>[2x]MPFTYSIEATRNLATTERCIQDIRNAPVRNRSTQFQLAQQNMLAYTFGEVIPGFASAGINGMDYRDVIGRPVENAVTEGTHFFRDDFRVDSNAKAKVAGDIFEIVSSAVMWNCAARWNSLMVGEGWRSQPRYSRPTLSPSPRRQVAVLNLPRSFDWVSLLVPESQEVIEEFRAGLRKDGLGLPTSTPDLAVVVLPEEFQNDEMWREEIAGLTRPNQILLSGAYQRLQGRVQPGEISLAVAFKRSLRSDRLYQPLYEANVMQLLLEGKLGAPKVEFEVHTLAPEGTNAFVTYEAASLYGLAEGRSAVHRAIRELYVPPTAADLARRFFAFLNERMELVNGENLYFQSHHHHHH

For the filament-forming sequence-specific DNA endonuclease SgrAI, the process of filamentation both accelerates its DNA cleavage activity and expands its DNA sequence specificity, thus allowing for many additional DNA sequences to be rapidly cleaved. Under basal conditions, SgrAI is a homodimeric and sequence-specific restriction endonuclease of 74 kDa with two active sites, one in each subunit. Each active site cleaves bound duplex DNA containing any one of 17 different 8 bp recognition sites. Three of these sites, known as primary sequences or primary sites, have the pattern CRCCGGYG (where R = A or G and Y = C or T) and can be cleaved by SgrAI in the absence of filamentation.

Second, we present an X-ray crystal structure of DNA-free (apo) SgrAI resolved to 2.0 Å resolution, which reveals a disordered loop involved in DNA recognition. To our surprise, we instead captured DNA-free SgrAI, without bound DNA. Two copies of the chain were found per asymmetric unit arranged with twofold symmetry to produce a complete SgrAI dimer in its apo form, which we refer to as SgrAIapo/DCA. The structure of SgrAIapo/DCA also contains a divalent metal ion. A single Ca2+ is found bound to each subunit near the active site, in the site designated as site D (see also Fig. S3B for the orientation of site D relative to sites A and B in SgrAISP/FCA). The Ca2+ bound to DNA-free SgrAI, SgrAIapo/DCA, is coordinated by six oxygen atoms arranged in an octahedral geometry, which are contributed by the side chains of Glu103 and Asn149, the main-chain carbonyl oxygens of Leu150 and Asp188, and two water molecules, respectively. The role of this divalent cation-binding site is not clear, although its occupancy in the DNA-free structures suggests it may serve as a reservoir for Mg2+ prior to DNA binding, because Mg2+ in sites A and B bridge the protein–DNA interface. Residues Asp22–Gln34 within a loop region are disordered in the absence of DNA.>[2x]MLFYSFFKTLIDTEVTVELKNDMSIRGILKSVDQFLNVKLENISVVDASKYPHMAAVKDLFIRGSVVRYVHMSSAYVDTILLADACRRDLANNKRQ;>[2x]GSMESAQAVAEPLDLVRLSLDEIVYVKLRGDRELNGRLHAYDEHLNMVLGDAEEIVTIFDDEETDKDKALKTIRKHYEMLFVRGDSVILIAPPRN;>[2x]MLPLTLLNATQGRPILVELKNGETFNGHLENCDNYMNLTLREVIRTMPDGDKFFRLPECYIRGNNIKYLRIQDEVLSQVAKQQAQQRENRGSRFRGRGQRGRGNYGHTAPNRRGRGRGGHMWSHPQFEK;>MSMTILPL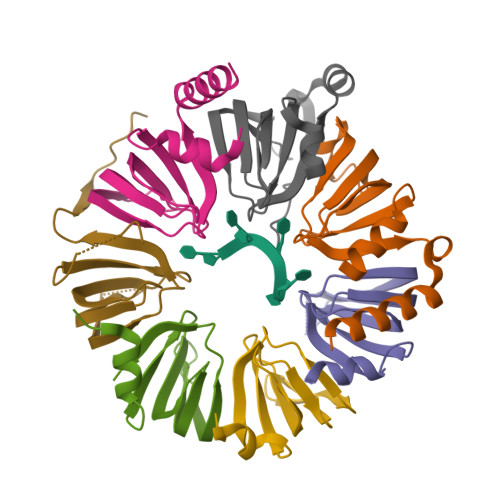ELIDKCIGSNLWVIMKSEREFAGTLVGFDDYVNIVLKDVTEYDTVTGVTEKHSEMLLNGNGMCMLIPGGKPE[2x];>[2x]GSMDSSPNEFLNKVIGKKVLIRLSSGVDYKGILSCLDGYMNLALERTEEYVNGKKTNVYGDAFIRGNNVLYVSALDD;>[2x]MSSLQKRPGPGNSSQPTERPRKESILDLSRYQDQRIQATFTGGRQITGILKGFDQLMNLVLDDVEEQLRNPEDGKLTGAIRKLGLVVVRGTTLVLIAPMDGSEEIPNPFVQAEHHHHHH;>[2x]MSLADFMEQRVQVITNDGRVVLGSLKGFDHTTNLILSDSFERIISMDQDMETIPLGVYLLRGENVAMVGLVNEELDSEIEWTKIRGEAIPDVVH Cilia and flagella-associated protein 410 (CFAP410) localizes at the basal body of cilia/flagella and plays essential roles in ciliogenesis, neuronal development and DNA damage repair. CFAP410 is a bimodular protein comprising two folded domains, i.e. NTD and CTD, which are connected through a variable unstructured loop. All these three crystal structures show a similar homotetrameric arrangement, with each monomer consisting of two α helices that form an open nutcracker-like conformation. Two CTDs first form an intercalated homodimer, and two such dimers further assemble into a tetramer by packing head-to-head through their first helices.

Homo sapiens CFAP410 (HsCFAP410) consists of 255 amino acids. The CTD truncations that finally generated well-diffracting crystals were fragments covering residues 256–295, 212–246 and 213–246 of H. sapiens, T. brucei and C. reinhardtii CFAP410 proteins, respectively. All HsCFAP410-CTD fragments were soluble in a buffer containing 20 mM HEPES (pH 7.5), 100 mM NaCl, and 1 mM DTT. The crystallizing condition for HsCFAP410-CTD contained 1.5 M NaCl and 10% (v/v) ethanol (22°C). Those of HsCFAP410-CTD and CrCFAP410-CTD were determined subsequently by molecular replacement using the crystal structure of TbCFAP410-CTD as a search template. One of the mutations, L224P, is located in the C-terminal domain (CTD) of human CFAP410 and causes severe spondylometaphyseal dysplasia, axial (SMDAX). Our results showed that for HsCFAP410-CTD both the wild-type and mutant A219E adopted the same conformation. However, the disease-causing mutant L224P lost all characteristic helical features and became completely unfolded. Our conformational analyses of the simulation data showed that while the wild-type model of HsCFAP410-CTD agreed very well with the crystal structure (all-atom RMSD = 0.8 Å), the simulated model of L224P was drastically different from the wild-type crystal structure, with the associated all-atom RMSD of 4.4 Å. The single-residue mutation L224P in HsCFAP410 that causes the autosomal recessive ciliopathy SMDAX may be attributed to the disrupted oligomeric assembly that causes the mislocalization of the protein possibly by abolishing its interaction with a partner protein at the basal body.

>[2x]GRNVLTAILLLLRELDAEGLEAVQQTVGSRLQA> SMTDLLSAEDIKKAIGAFTAADSFDHKKFFQMVGLKKKSADDVKKVFHILDKDKDGFIDEDELGSILKGFSSDARDLSAKETKT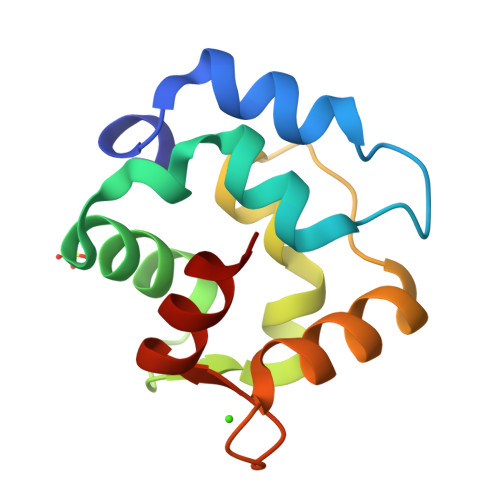LMAAGDKDGDGKIGVEEFSTLVAES> MKPHPWFFGKIPRAKAEEMLSKQRHDGAFLIRESESAPGDFSLSVKFGNDVQHFKVLRDGAGKYFLWVVKFNSLNEL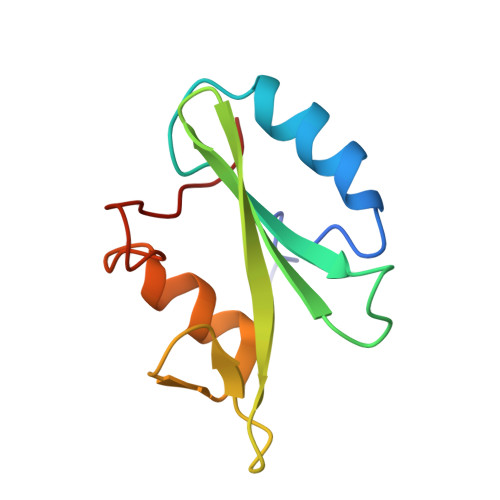VDYHRSTSVSRNQQIFLRDIE8-BROMOGUANINE | C5 H4 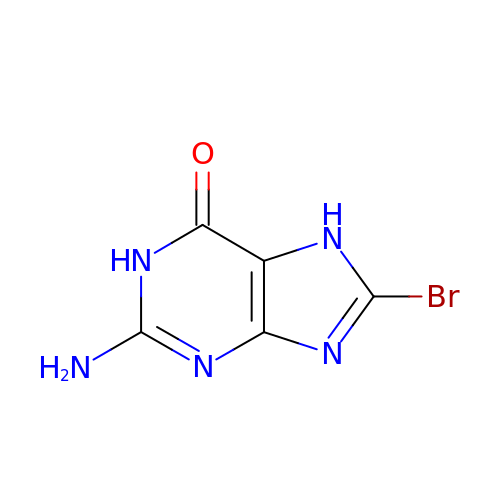Br N5 O | CRYCZDRIXVHNQB-UHFFFAOYSA-N>[4x]MKPQVYHVDAFTSQPFRGNSAGVVFPADNLSEAQMQLIARELGHSETAFLLHSDDSDVRIRYFTPTVEVPICGHATVAAHYVR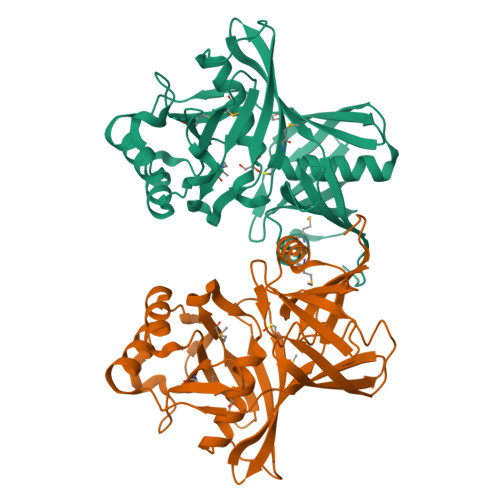AKVLGLGNCTIWQTSLAGKHRVTIEKHNDDYRISLEQGTPGFEPPLEGETRAAIINALHLTEDDILPGLPIQVATTGHSKVMIPLKPEVDIDALSPDLNALTAISKKIGCNGFFPFQIRPGKNETDGRMFSPAIGIVEDPVTGNANGPMGAWLVHHNVLPHDGNVLRVKGHQGRALGRDGMIEVTVTIRDNQPEKVTISGTAVILFHAEWAIEL pmcHuman ornithine aminotransferase (hOAT) is an enzyme that catalyzes the transfer of the δ-amino group from l-ornithine (l-Orn) to α-ketoglutarate (α-KG). As a pyridoxal-5′-phosphate (PLP)–dependent transaminase, hOAT has a “Bi−Bi, Ping–Pong” kinetic mechanism. In the first half-reaction, PLP and l-Orn are converted to pyridoxamine phosphate (PMP) and l-glutamate-γ-semialdehyde (l-GSA). l-GSA is then prone to cyclize to Δ1-pyrroline-5-carboxylate (P5C). In the second half-reaction, hOAT catalyzes the transfer of the amino group of PMP to an α-keto acid, preferentially α-KG, forming glutamate and regenerating the PLP form of the cofactor.

For GABA, an intermediate formed that exhibited a covalent linkage with PLP and was detached from the catalytic Lys292, a structure consistent with the proposed external aldimine intermediate. The carboxylate group of the ligand formed two hydrogen bonds with Tyr55 instead of interacting with Arg180, which is proposed to interact with the carboxylate of l-Orn. No other interactions were observed between the ligand and the active-site residues. For two monomer copies in an asymmetric unit, the Glu235–Arg413 salt bridge that is a key feature in the holo-hOAT was found partially disrupted: the side chain of Arg413 moved away from Glu235 and Gln266. In other monomer copies, the Glu235–Arg413 salt bridge remained intact. The salt bridge in the GABA structure was found disrupted in two of six monomers in an asymmetric unit. It is possible that the salt bridge could be broken during the first half-reaction to prepare the enzyme for the second half-reaction. Considering the exceedingly slow reaction rate, relatively short soaking time, and good fit of the model into the observed electron density, it can be concluded that the species observed in the structure is not a final adduct but rather an external aldimine intermediate. However, considering the transient-state data, the external aldimine appears to be the most probable reaction intermediate to be observed in the crystal structure. By contrast, the external aldimine is free from Lys292 and is distanced 3.4 Å from its ε-amino group.

>[6x]MFSKLAHLQRFAVLSRGVHSSVASATSVATKKTVQGPPTSDDIFEREYKYGAHNYHPLPVALERGKGIYLWDVEGRKYFDFLSSYSAVNQGHCHPKIVNALKSQVDKLTLTSRAFYNNVLGEYEEYITKLFNYHKVLPMNTGVEAGETACKLARKWGYTVKGIQKYKAKIVFAAGNFWGRTLSAISSSTDPTSYDGFGPFMPGFDIIPYNDLPALERALQDPNVAAFMVEPIQGEAGVVVPDPGYLMGVRELCTRHQVLFIADEIQTGLARTGRWLAVDYENVRPDIVLLGKALSGGLYPVSAVLCDDDIMLTIKPGEHGSTYGGNPLGCRVAIAALEVLEEENLAENADKLGIILRNELMKLPSDVVTAVRGKGLLNAIVIKETKDWDAWKVCLRLRDNGLLAKPTHGDIIRFAPPLVIKEDELRESIEIINKTILSF> ASQPPQVTVDKLKRLENDFGGRIGVYAIDTGSNKTFGYRANERFPLCASFKGFLAAAVLSKSQQQEGLLNQRIRYDNRVMEPHSPVTEKQITTGMTVAELSAATLQYSDNGAANLLLEKLIGGPEGMTSFMRSIGDNVFRLDRWELELNSAIPGDDRDTSTPKAVAESMQKLAFGNVLGLTERHQLMDWFKGNTTGGARIRASVPANWVVGDKTGTCGVYGTAND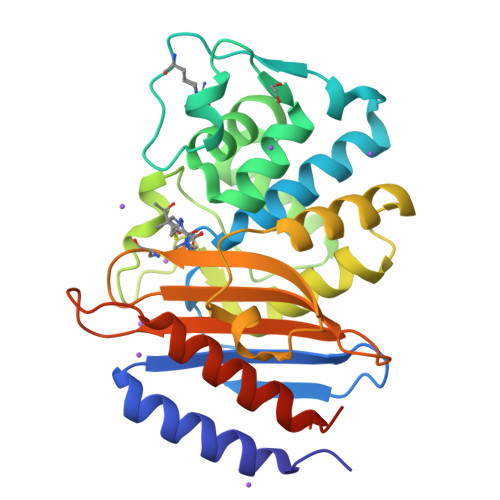YAVIWPVAHAPIVLAVYTSKPDRNSKHSDAVIADASRIVLESFNIDALRMATGKSIGF>FYKREMFDPAEEYKMNHKRRGLALIFNQKRFDWKLGLKTRNGTDKDRDNLERRFQELGFEVKAYNDLS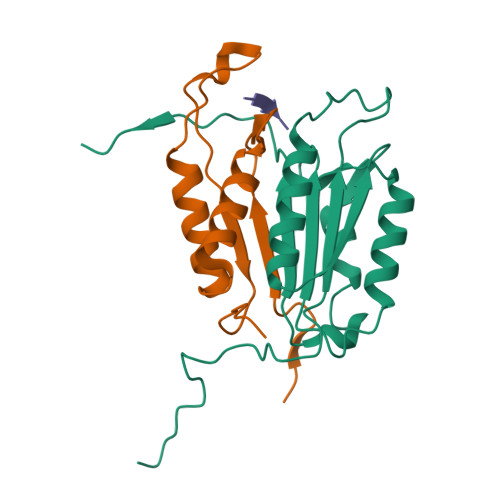AEEVLEKIQEASTADHSDADCFVCVFLSHGEDGHVYANDAKIEIQELTNLFKGDKCQSLVGKPKIFIIQACRGDKLDDAVTPM[4x];>VYTLPAGADFIMCYSTAEGYYSYRETVNGSWYIQDLCEMLKKYGSELEFTEILTLVNRKVSLRSVPNCKDPAAIGKKQMPCFASMLTKKLYFRPK[4x];>VEID[4x]>MTRTLPPGVSDERFDAALQRFRDVVGDKWVLSTADELEAFRDPYPVGAAEANLPSAVVSPESTEQVQDIVRIANEYGIPLSPVSTGKNNGYGGAAPRLSGSVIVKTGERMNRILEVNEKYGYALLEPGVTYFDLYEYLQSHDSGLMLDCPDLGWGSVVGNTLDRGVGYTPYGDHFMWQTGLEVVLPQGEVMRTGMGALPGSDAWQLFPYGFGPFPDGMFTQSNLGIVTKMGIALMQRPPASQSFLITFDKEEDLEQIVDIMLPLRINMAPLQNVPVLRNIFMDAAAVSKRTEWFDGDGPMPAEAIERMKKDLD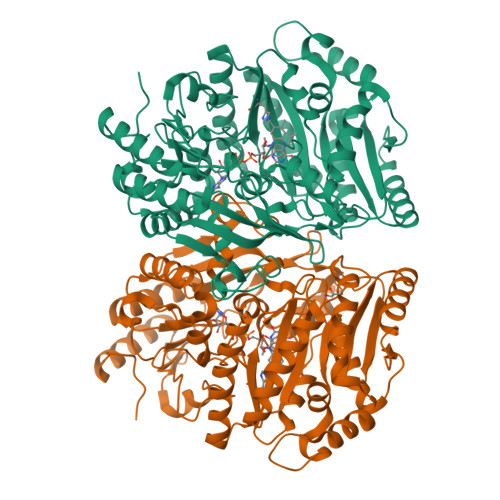LGFWNFYGTLYGPPPLIEMYYGMIKEAFGKIPGARFFTHEERDDRGGHVLQDRHKINNGIPSLDELQLLDWVPNGGHIGFSPVSAPDGREAMKQFEMVRNRANEYNKDYAAQFIIGLREMHHVCLFIYDTAIPEAREEILQMTKVLVREAAEAGYGEYRTHNALMDDVMATFNWGDGALLKFHEKIKDALDPNGIIAPGKSGIWSQRFRGQNL[2x]>MGKRMVVVGGVAGGASAAAKAKRENPELEVVVYEKSGWVSYGACGLPYVLSGEIPRLERLVARTPEEFRKQGVLVHTRHEVVDVDYELRTLTVHDHAEGRTFQDRFDHLVLATGARPSLPPIPGTEQEGVYTLRTMEDGERLLKALPQARRAAILGAGYIGLEAAEAFRKRGLQVTLLEAKDRPLPHWDPEVGALLKEELERHGVEVWTGVKVEAFRGMGRVEAVETSEGVVPADLVLLATGIRPNTELAQAMGVALGPTGAIATDERMRTNLEGVYAAGDVAESFHRVLKRPYWLPLGDVANKHG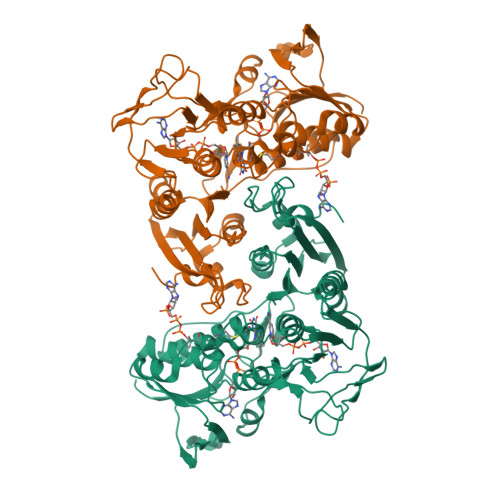RTAGSVIAGREARFLGVVGTAIFKAFDLAVATTGLSLEGALKEGFWAKKVFIQSRDGAHYYPGSGPLWVELVYEEGTGRLLGGAVVARGHGALRIDVLAALLHREGSVEDLLALDLAYAPPFSPVWDPLLIAAQQAR[4x]>SPPKPKCRCGISGSSNTLTTCRNSRCPCYKSYNSCAGCHCVGCKNPHKEDYV[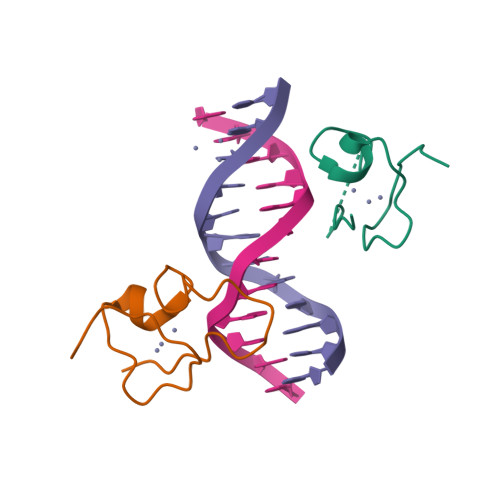2x]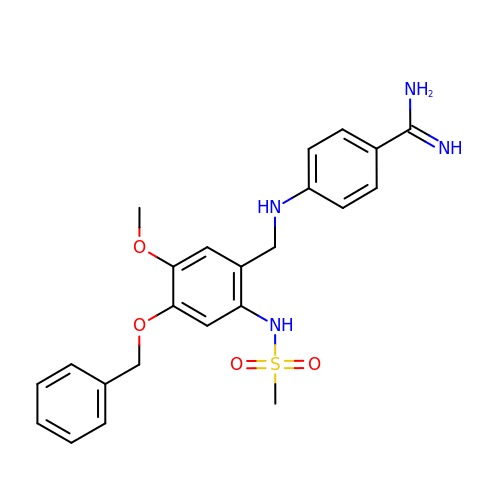4-(4-BENZYLOXY-2-METHANESULFONYLAMINO-5-METHOXY-BENZYLAMINO)-BENZAMIDINE | C23 H26 N4 O4 S | CRFICMUDNBIMKL-UHFFFAOYSA-N> SHFN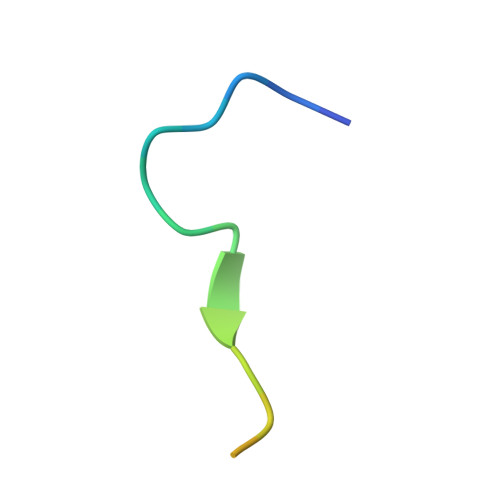LAPLGRRRVQSQWASTR>MAKETKKRAPRKRLTPFQKQAHNKIEKRYRININTKIARLQQIIPWVASEQTAFEVGDSVKKQDEDGAETAATTPLPSAAATSTKLNKSMILEKAVDYILYLQNNERLYEMEVQ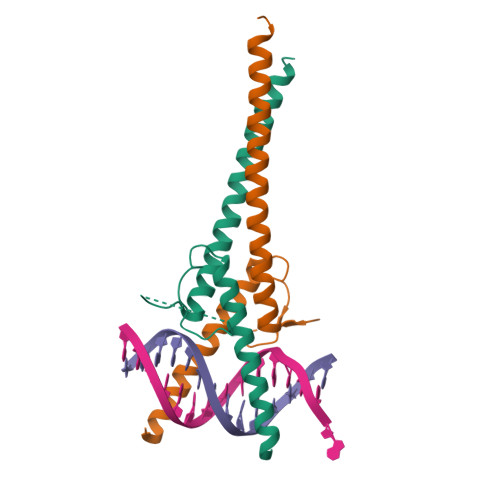RLKSEIDTLKQDQKLEHHHHHH[2x]>ANQLAKDLEIMFENYVEGFEAACVVSRNAKKFRPGDTAMQRAGDVLYRPQHYHMNIEEGLDLSSKTPTALVQRLVPSVFKEPKNILYTLDAREMRDPEHKTEAGRAAGMRLAAQIDSDLISMVTQRATNVITMADSTAGTQGRDLWNCAAGIDATMTAIGVPQGINRRSFWNPFNYKDLAGELGHRAYAQGATLTAYEKAQIPPVASFDSYKTDISGRLPKGSTESLTVSGQPEHKVEAKDSNGMPVDNRQGTITVSASGLQVGDAFTIAGVNSVHQITK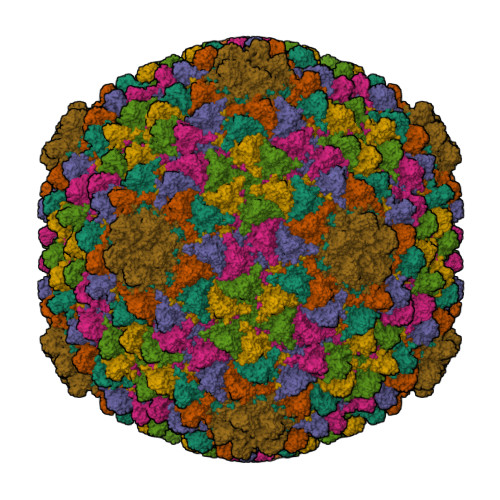DTTGQPQVFRVLAVSGTTVTISPKILPVENTDVASRPYANVDAKPAESAAITILNKNAAPANLFWADGSVELMYGKLAFPTGQGPQVMTATTEQGATLIMSYAFDHIKGVTTARFTTLYGCSVLVPEYTGIVIAGQ[7x]(2R)-3-[(2E,6E)-3,7,11-trimethyldodeca-2,6,10-trienoxy]propane-1,2-diol | C18 H32 O3 | 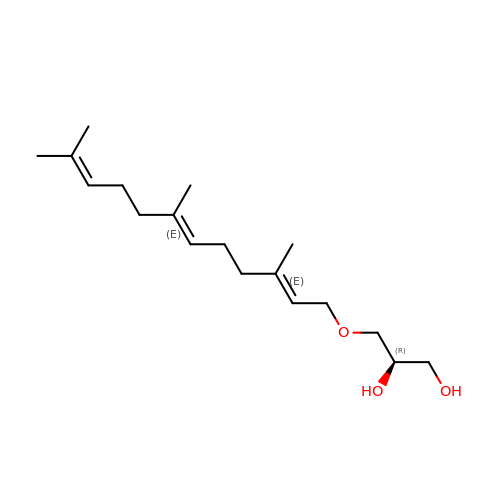VGIZXGYRSPTVQF-LEAVJPGDSA-N> MSLNVSRLLLPSRVRHSYTGKMGAVFIFVGALTVLFGAIAYGEVTAAAATGDAAAVQEAAVSAILGLIILLGINLGLVAATLGGDTAASLSTLAAKASRMGD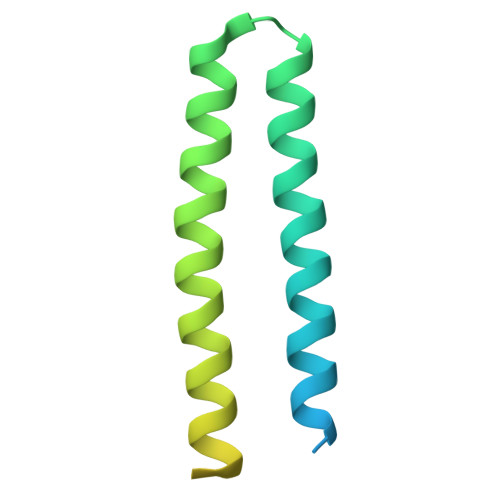GDLDVELETRREDEIGDLYAAFDEMRQSVRTSL>MRVIFSEDHKLRNAKTELYGGELVPPFEAPFRAEWILAAVKEAGFDDVVAPARHGLETVLKVHDAGYLNFLETAWDRWKAAGYKGEAIATSFPVRRTSPRIPTDIEGQIGYYCNAAETAISPGTWEAALSSMASAIDGADLIAAGHKAAFSLCRPPGHHAGIDMFGGYCFINNAAVAAQRLLDKGAKKIAILDVDFHHGNGTQDIFYERGDVFFASLHGDPAEAFPHFLGYAEETGKGAGAGTTANYPMGRGTPYSVWGEALTDSLKRIAAFGAEAIVVSLGVDTFEQDPISFFKLTSPDYITMGRTIAASGVPLLVVMEGGYGVPEI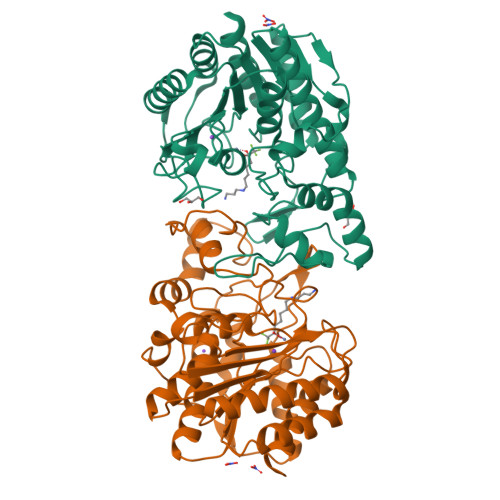GLNVANVLKGVAG[2x]> WNIGKLIYMDNISPEECIRRWRGEDDDSKDESDIEEDVD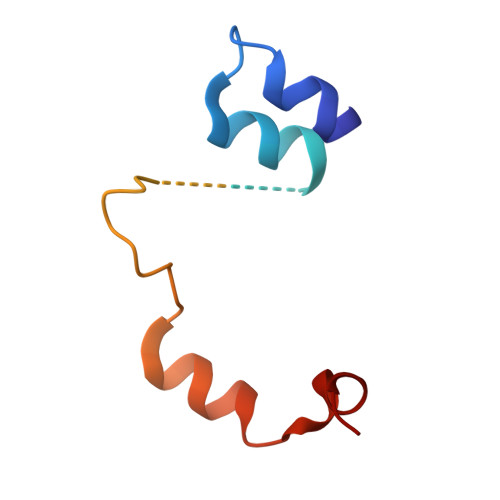DDFFRKKDGTVTKEGNKDHAVDLEKFVPYFDTFEKLAKKWKSVDAIKERFL>[2x]MPLCTLRQMLGEARKHKYGVGAFNVNNMEQIQGIMKAVVQLKSPVILQCSRGALKYSDMIYLKKLCEAALEKHPDIPIC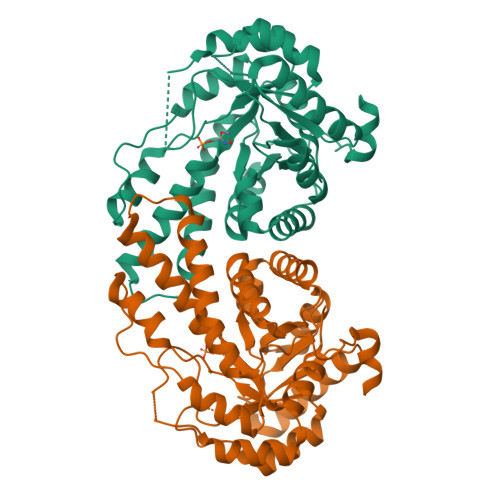IHLDHGDTLESVKMAIDLGFSSVMIDASHHPFDENVRITKEVVAYAHARSVSVEAELGTLGGIEEDVQNTVQLTEPQDAKKFVELTGVDALAVAIGTSHGAYKFKSESDIRLAIDRVKTISDLTGIPLVMHGSSSVPKDVKDMINKYGGKMPDAVGVPIESIVHAIGEGVCKINVDSDSRMAMTGAIRKVFVEHPEKFDPRDYLGPGRDAITEMLIPKIKAFGSAGHAGDYKVVSLEEAKAWYK3-(3,4-dihydroisoquinolin-2(1H)-yl)propan-1-amine | C12 H18 N2 | 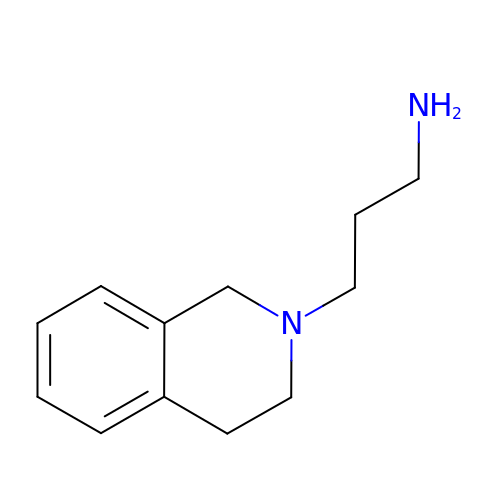OZWGXKVQFUBMTE-UHFFFAOYSA-N> MSLGPLWLDVAGYELSAEDREILQHPTVGGVILFGRNYHDNQQLLALNKAIRQAAKRPILIGVDQEGGRVQRFREGFSRIPPAQYYARAENGVELAEQGGWLMAAELIAHDVDLSFAPVLDMGFACKAIGNRAFGEDVQTVLKHSSAFLRGMKAVGMATTGKHFPGHGAVIADSHLETPYDERETIAQDMAIFRAQIEAGVLDAMMPAHVVYPHYDAQPASGSSYWL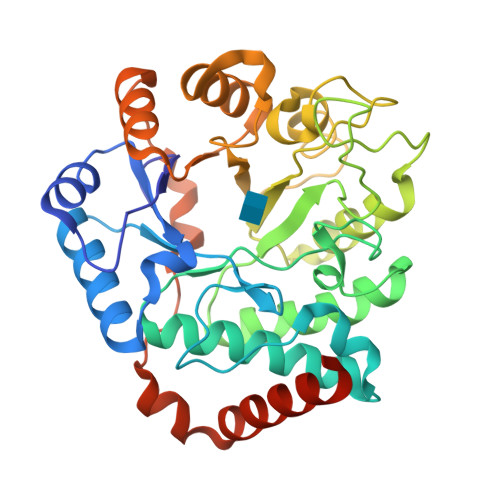KQVLREELGFKGIVFSDDLSMEGAAVMGGPVERSHQALVAGCDMILICNKREAAVEVLDNLPIMEVPQAEALLKKQQFSYSELKRLERWQQASANMQRLIEQFSEEGGSHHHHHH>SNAMNRSNIWNLLFTILIIVTLFWLARFFYVENSPVSKLSYTSFVQMVEDERSVVSEVVIRDDGVLRVYTKDGRVYEVDAPWAVNDSQ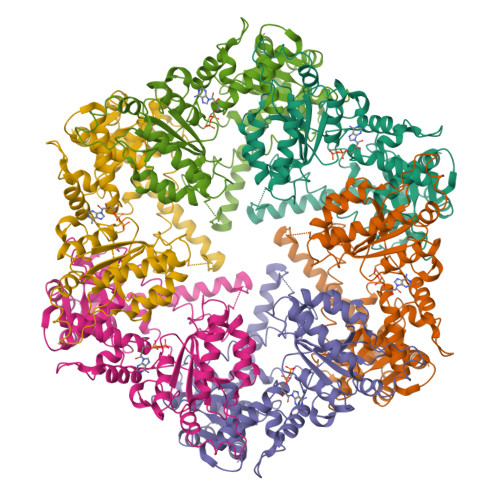LIEKLVSKGIKVSGERSGSSSFWINVLGTLIPTILFIVVWLFIMRSLSGRNNQAFTFTKSRATMYKPSGNKRVTFKDVGGAEEAIEELKEVVEFLKDPSKFNRIGARMPKGILLVGPPGTGKTLLARAVAGEANVPFFHISGSDFVELFVGVGAARVRDLFAQAKAHAPCIVFIDEIDAVGRHRGAGLGGGHDEREQTLNQLLVEMDGFDSKEGIIVMAATNRPDILDPALLRPGRFDKKIVVDPPDMLGRKKILEIHTRNKPLAEDVNLEIIAKRTPGFVGADLENLVNEAALLAAREGRDKITMKDFEEAIDRVIAGPARKSKLISPKEKRIIAYYEAGHAVVSTVVPNGEPVHRISIIPRGYKALGYTLHLPEEDKYLVSRNELLDKLTALLGGRAAEEVVFGDVTSGAANDIERATEIARNMVCQLGMSEELGPLAWGKEEQEVFLGKEITRLRNYSEEVASKIDEEVKKIVTNCYERAKEIIRKYRKQLDNIVEILLEKETIEGDELRRILSEEFEKVVE[6x]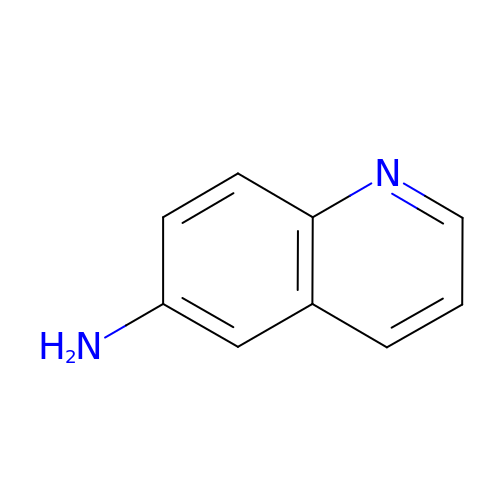quinolin-6-amine | C9 H8 N2 | RJSRSRITMWVIQT-UHFFFAOYSA-N> GGLEKDFLPLYFGWFL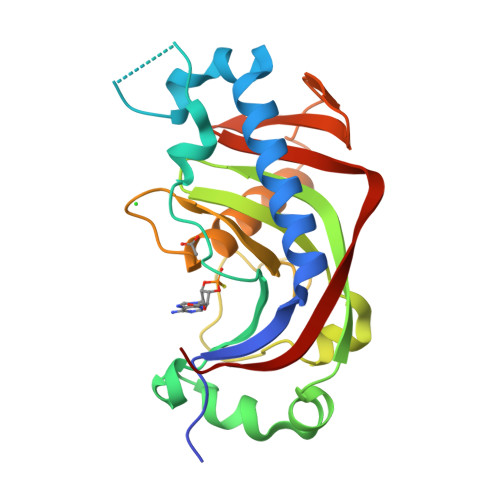TKKSSETLRKAGQVFLEELGNHKAFKKELRHFISGDEPKEKLELVSYFGKRPPGVLSCTTKFCDYGKAAGAEEYAQQEVVKRSYGKAFKLSISALFVTPKTAGAQVVLTDQELQLWPSDLDKPSASEGLPPGSRAHVTLGCAADVQPVQTGLDLLDILQQVKGGSQGEAVGELPRGKLYSLGKGRWMLSLTKKMEVKAIFTGYYG>[2x]GTMARNDGQGKAAATFMHISYNNFITEVDNLNKRMGDLRDINGEAGTWVRLLNGSGSADGGFTDHYTLLQMGADRKHELGSMDLFTGV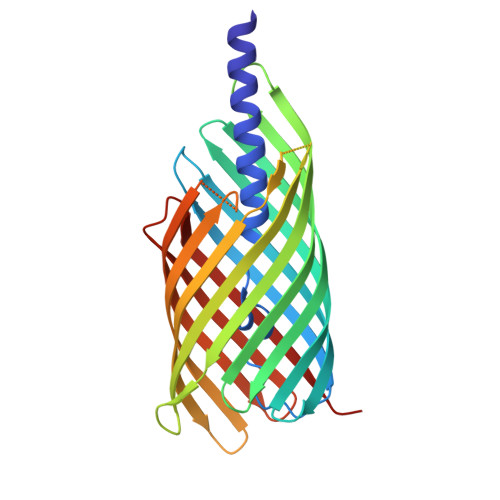MATYTDTDASADLYSGKTKSWGGGFYASGLFRSGAYFDVIAKYIHNENKYDLNFAGAGKQNFRSHSLYAGAEVGYRYHLTDTTFVEPQAELVWGRLQGQTFNWNDSGMDVSMRRNSVNPLVGRTGVVSGKTFSGKDWSLTARAGLHYEFDLTDSADVHLKDAAGEHQINGRKDSRMLYGVGLNARFGDNTRLGLEVERSAFGKYNTDDAINANIRYSFLE> MKSKFKLTTAAAMLGLMVLAGGAQAQDKPREVLTGGHSVSAPQENRIYVMDSVFMHLTESRVHVYDYTNGKFLGMVPTAFNGHVQVSNDGKKIYTMTTYHERITRGKRSDVVEVWDADKLTFEKEISLPPKRVQGLNYDGLFRQTTDGKFIVLQNASPATSIGIVDVAKGDYVEDVTAAAGCWSVIPQPNRPRSFMTICGDGGLLTINLGEDGKVASQSRSKQMFS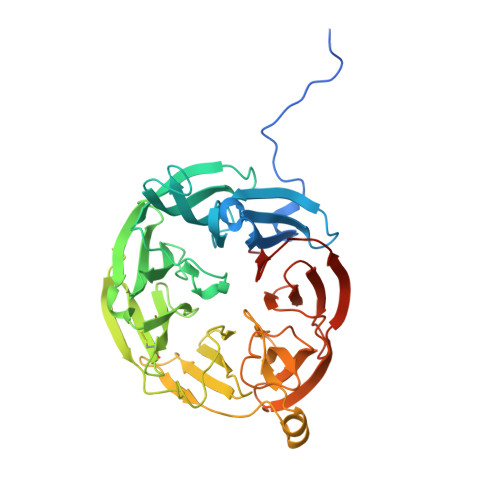VKDDPIFIAPALDKDKAHFVSYYGNVYSADFSGDEVKVDGPWSLLNDEDKAKNWVPGGYNLVGLHRASGRMYVFMHPDGKEGTHKFPAAEIWVMDTKTKQRVARIPGRDALSMTIDQQRNLMLTLDGGNVNVYDISQPEPKLLRTIEGAAEASLQVQFHPVGGV9-[(2~{R},3~{R},4~{S},5~{R})-3,4-bis(oxidanyl)-5-[[tris(oxidanyl)-$l^{5}-phosphanyl]oxymethyl]oxolan-2-yl]-2-oxidanyl-1~{H}-purin-6-one | C10 H13 N4 O9 P 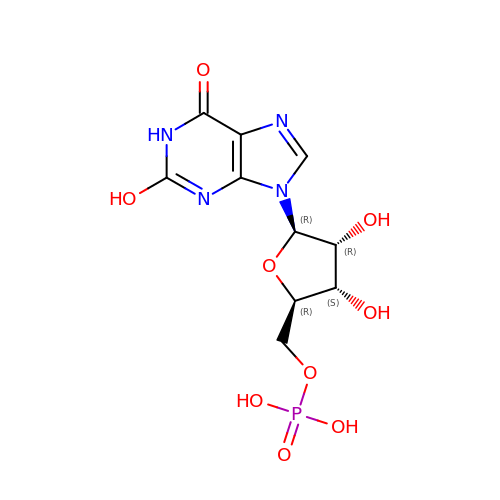| DCTLYFZHFGENCW-UUOKFMHZSA-N> MAHHHHHH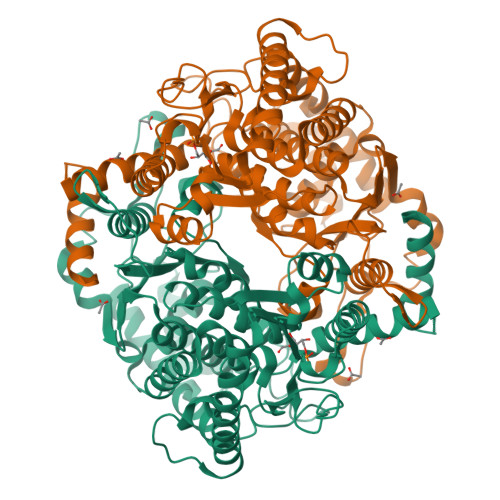MMGKGFLDCESLVALQEMALHPIDLTASGCLSEERIQKNSLSVEGFTYSYATERVDDRCLEALQGLTEERELIKQMECMQQGAIMNRIEGFQSESRPVLHTATRAWVRDQDLHEEAAAIARHSKEEALRLAEFLYIARAKFSTLVQIGIGGSELGPKAMYFAMQGSCPSDKRIFFVSNIDPDNAAEVLREIDLEQTLVVVVSKSGTTLEPAANEELFRQAYQNKGLSIAEHFVAVTSQGSPMDDKSRYLEVFHLWDSIGGRFSATSMVGGVVLGFAFGYEAFIEFLQGAAAIDAHALTPKMRENLPLLSAMLGVWNRNLLGYPTTAVIPYSTGLKYFTAHLQQCGMESNGKSISREGKEISFRTSPIIWGDVGTNCQHSFFQSLHQGTDIVPVEFIGFLHNQRGLDCVLSGSSSSQKLFANLVAQSLALAQGRDNANPNKRFKGNSPSSILVAQQLSPRIAGSLLAFYEHKFAFQGFCWGINSFDQEGVSLGKELATQIIGIMSGNAPVEFPEARGVLRLFNVLT>[2x]TALTNLVAEPFAKLEQDFGGSIGVYAMDTGSGATVSYRAEERFPLCSSFKGFLAAAVLARSQQQAGLLDTPIRYGKNALVPWSPISEKYLTTGMTVAELSAAAVQYSDNAAANLLLKELGGPAGLTAFMRSIGDTTFRLDRWELELNSAIPGDARYTSSPRAVTESLQKLTLGSALAAPQRQQFVDWLKGNTTGNHRIRAAVPADWAVGDKTGT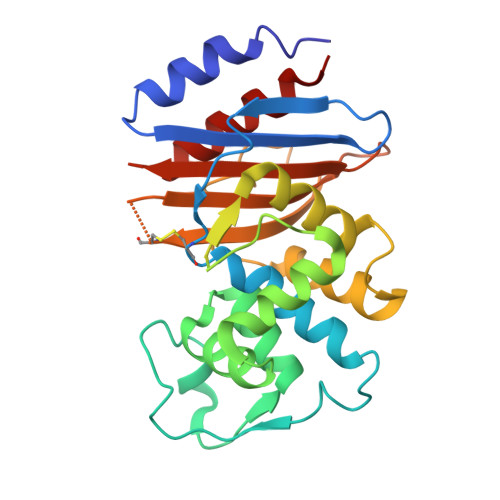CGVYGTANDYAVVWPTGRAPIVLAVYTRAPNKDDKHSEAVIAAAARLALEGLG> MQRKGTDEIYGLGSLPSAGPGRWEYLANPGNWHPERRKLHEKLLDQARSSALTLAESLESDGCQPTLFALRGNTATGKTRIATKKIPVLAAALKKTAGKGCVNPDVFKSSLAKSETGAKIFSSAQVHSESSFLADRFEGGLRSQKTGSGAIASIVVDKRLSREYEIDSYIQLAKETGRKVELCDIDAPLENSLVGVLQRKPEGEDPRPPYPVVSSGFVAVRSNRMYVIDRFIADPSLGNYRLFGTAEDGEKVMVASVIGGEFSVENAELYEKITSPQLSVTGDLADKVIDKELIDRLENNIAD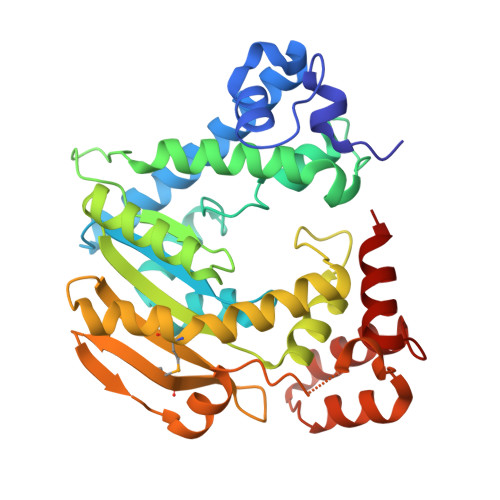PERAAKTRAALEKYSGKSWSAALAAHSELI> MRDVAIIGYGQTKFGELWEDSFRDLIVEAGVKAIKDANVDGGDIDAMYIGNMSGGLFVGQEHIASLIADHAGLNPVPCTRVEAACASGSLALRSAVLSVASGHHDVVLAGGVE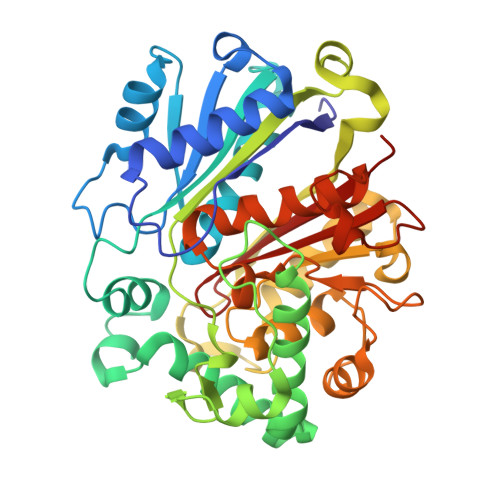KMTDVEDATAAIASASDQEWEAFFGATFPSLYAMMARRYMYQYGLTIEELSMWSVIAHENATKNKYAQFGFKTTLEQVMNASPVADPLTLMHCSPVSDGASALIVCDADKAEEFAPKDEIIYIKASTQASDTIALHDREDMTTLNAAKVASEKAYKLAKIAPEKIDVAEVHDCFAINGLILVEDLGFCKKGDAGKVIDEGKIRIDYDDFVTVNPSGGLKAAGHALGATGIRQVGELYWQLKQDKECKDRQATIKNGYGIAANVGGTGGTVCVHLLSDKR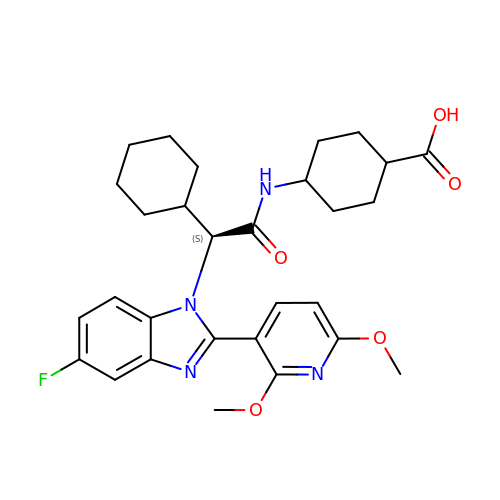trans-4-({(2S)-2-cyclohexyl-2-[2-(2,6-dimethoxypyridin-3-yl)-5-fluoro-1H-benzimidazol-1-yl]acetyl}amino)cyclohexane-1-carboxylic acid | C29 H35 F N4 O5 | JHVYRIYZUSZRSR-KHOMTPLRSA-N> GGGHMI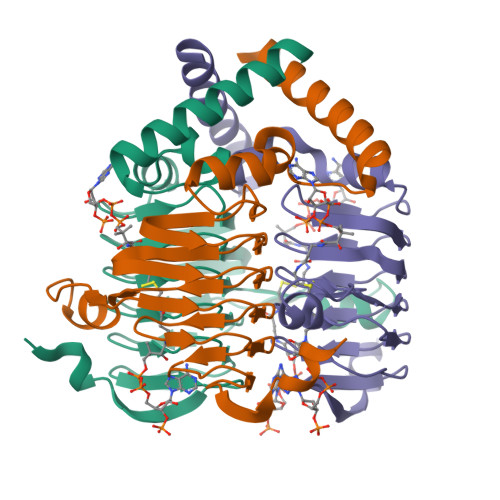LLKELKELFFLRTTYYLKKYNRSLPFGDMIVDRWDKAKLLGFGEGTSIYDSSIVLGEVKVGKDTWIGPNTILDGSGGGLIIGSNCSISAGVQIYTHDTVRKSLSGGKADIDKASTRIGSDCYLGPNTIIVKGVKIGDRVVVGANSLVLKDIPSDCKVFGSPAVIITDSLNYQRNNI>GAGSTAGKVIKCKAAVLWEEKKPFSIEEVEVAPPKAHEVRIKMVATGICRADDHVVSGTLVTPLPVIAGHEAAGIVESIGEGVTTVRPGDKVIPLFTPQCGKCRVCKHPEGNFCLKNDLSMPRGTMQDGTSRFTCRGKPIHHFLGTSTFSQYTVVDEISVAKIDAASPLEKVCLIGCGFSTGYGSAVKVAKVTQGSTCAVFGLGGVGLSVIMGCKAAGAARIIGVDINKDKFAKAKEVGATECVNPQDYKKPIQEVLTEMSNGGVDFSFEVIGRLDTM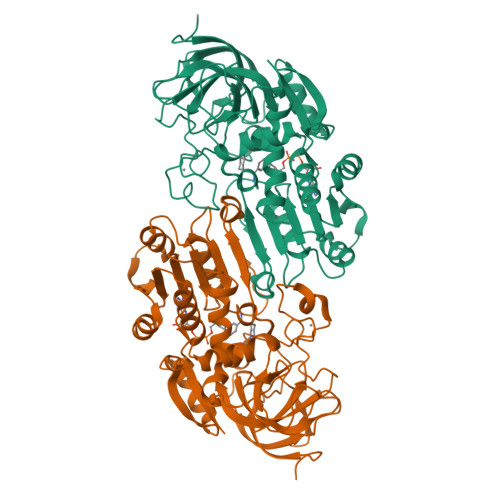VTALSCCQEAYGVSVIVGVPPDSQNLSMNPMLLLSGRTWKGAIFGGFKSKDSVPKLVADFMAKKFALDPLITHVLPFEKINEGFDLLRSGESIRTILTF[4x]>[2x]MGSMLSFILTLKRMLKACLRAWKDKEFQVLFVLTFLTLTSGTIFYSTVEGLRPLDALYFSVVTLTTVGDGNFSPQTDFGKVFTI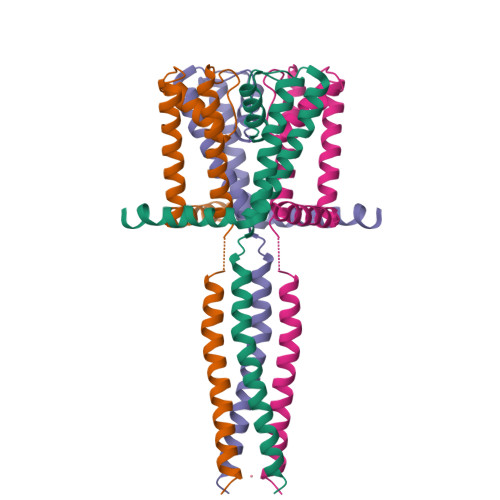LYIFIGIGLVFGFIHKLAVNVQLPSILSNRKKETDAYRLEVMEKLEAIEKKLAEHSRQGSLVPR> TEAQ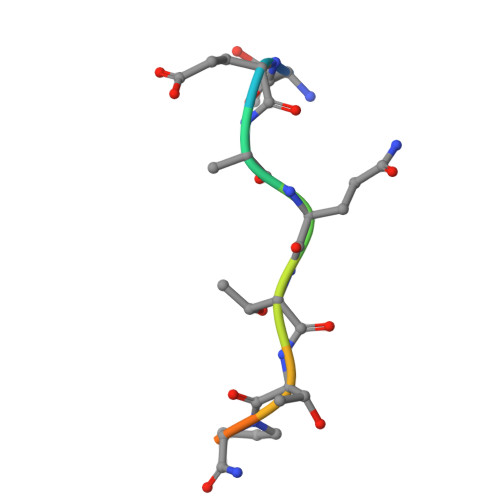TTPPPA>[2x]GSAKDPMLYIYIKTQNALVQRINFNLDSQELPQNILWIDLLHPSAAEIAFISSEFNLEFPTKEEREEIELSAKYWEDNATITINAHFLVRDLKSDEEDRNLIKLRTEIVTFATAKNILFTIRYNEFSTFEEIQARILASPKNFEDGFDIIDKMFEVRVEKDADLLEWIDKEARRLRTSVLEKKDEYSYDEM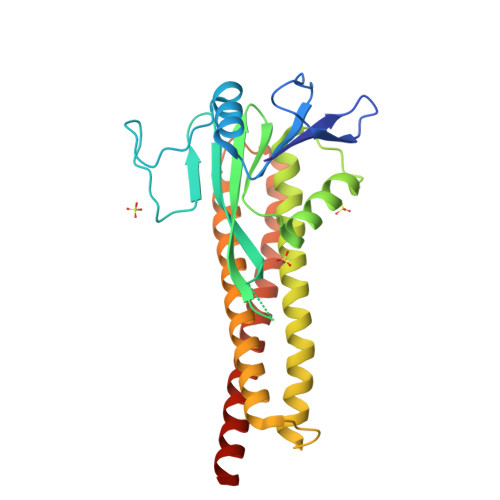LKDISSLQELNMRVRDSLFDKRRAMTSLLKSDKIDKDIKQNLTIVLKDLNSLVEFSVSQLNILDNIQTILASQINIEQNKIIK The viral nucleoprotein (NP), a key component of the replication machinery, packages the viral genome into protective ribonucleoprotein particles. Although TiLV-NP is considerably smaller than its influenza counterpart and unrelated in sequence, it maintains the same topology and domain organisation. This comprises a head and body domain between which is a positively charged groove, where single-stranded RNA binds. In addition, an oligomerisation loop inserts into a hydrophobic pocket in the neighbouring NP, the flexible hinges of which allow variable orientation of adjacent NPs.

In addition to the two tetramers, pentameric and hexameric oligomers were also resolved, displaying pseudo-C5 and pseudo-C6 symmetries. These higher-order oligomers resemble the pseudo-C4 structure but incorporate additional NPs, resulting in circular assemblies with diameters of ∼107 Å for the pentamer and ∼122 Å for the hexamer. The NP–NP interface areas are smaller, averaging 1240 Å² for the pentamer and 1065 Å² for the hexamer. The pseudo-C2 and pseudo-C5 oligomers appeared the most stable with uniform density according to local resolution, while the pseudo-C4 and pseudo-C6 structures displayed poorer density for 2 and 3 NPs, respectively. In the pseudo-C5 oligomers, up to 12 nucleotides can be modelled per NP. The RNA-binding mode is conserved across all NPs, with ∼930 Å2 of RNA surface buried within each groove, making the RNA largely inaccessible to the solvent. Only discontinuous RNA density is observed at the NP–NP interfaces suggesting two potential binding modes: either individual vRNA loops interact separately with each NP, or a single vRNA loop may bridge two adjacent NPs, leaving a flexible RNA loop at the NP-NP interface. Assuming TiLV-RNPs adopts an anti-parallel superhelix like influenza, it is tempting to suggest that the circularised TiLV-NP pentamers and hexamers may correspond to the loop found at one extremity of the RNP or could, perhaps, correspond to a nascent RNP formed within the replication complex once the RNA product begins to bulge out.

>[5x]MVRTTKTSMAAASTVAPEVAMDEGSPSTSQAQVELPRNLEVFNEACGHVFGSSFNREDNSVISDAAAFLFKMHTHSLDGQEAKVLRASEKKRERENAKKSRKAPEAGMRVGRSLILTSRWTEYCATCVPALGSKMKVIKASGDAAMIQMMKDHNSLLRVCVRIEVWKARYVSLVALDERIQTLEDAQWFPYLSGDSYRACPGLVGGYFAKKAAAGERGKNYKKLNQTAIIPPPRFLIIGHRLQIGDQVTLRELLASIAWGLCDGVLAECWSPSQGDGSIGVVVGLPLQATGSCFLVVASHGLSAIADSRIEGTGNTNLLEECIAIQKQDGVIKCKRSGKSLYHCLKETAGAVGR ACBD3 is a Golgi resident protein involved in the maintenance of the Golgi structure and regulation of intracellular trafficking between the endoplasmic reticulum and the Golgi. However, in enterovirus-infected cells, the ACBD3 GOLD domain interacts preferentially with viral non-structural 3A proteins, which causes re-localization of ACBD3 to the sites of virus replication. In this study, we present a structural, biochemical, and biological characterization of the complexes composed of human ACBD3 and the 3A proteins of four representative enteroviruses. The crystal structures revealed the details of the ACBD3-3A interaction, the 3A-3A interaction causing the assembly of the ACBD3-3A heterotetramers, the interaction between the ACBD3-3A complex and the lipid bilayer, and the roles of these interactions in facilitation of enterovirus replication.

To ensure that the 3A protein is fully complexed with the ACBD3 GOLD domain and to avoid the formation of partial complexes with 1:2 stoichiometry, we designed a GOLD-EVD68 3A fusion protein using a similar approach as for the GOLD-EVA71 3A fusion protein used for the crystallographic analysis. Taking advantage of the vicinity of the C terminus of the ACBD3 GOLD domain and the N terminus of the ordered part of the EVD68 3A protein, we connected the last residue of ACBD3 (R528ACBD3) through a short peptide linker (GSGSG) to the first ordered residue of the EVD68 3A protein (T163A/EVD68). Both GOLD-3A wild-type and LVVY mutant fusion proteins formed crystals, which diffracted to a resolution suitable for further structure determination. The crystal structures of the GOLD: 3A complex consisting of two individual proteins, the GOLD-3A fusion protein, and its LVVY mutant were almost identical with low root-median-square deviations, confirming that neither the fusion-protein approach nor the LVVY mutation affected the correct folding of these proteins. Three lines of evidence document the dimeric state of the wild-type GOLD-3A fusion protein and the monomeric state of its LVVY mutant in vitro. First, the retention volumes of these proteins in size exclusion chromatography are significantly shifted. Secondly, the small-angle X-ray scattering (SAXS) profiles of these proteins correspond to the calculated scattering curves of a dimer of the wild-type GOLD-3A fusion protein and of a monomer of its LVVY mutant. Nevertheless, we observed a significant difference in FRET efficiency between the wild-type GOLD-3A fusion protein and its LVVY mutant. These results confirm that the GOLD: 3A complexes are flexible enough to allow the formation of the heterotetramers consisting of two molecules of the viral 3A protein and two molecules of host ACBD3 even in cells at the respective intracellular membranes.

> GAMESLPVIAAPSMWTRPQIKDFKEKIQQDADSVITVGRGEVVTVRVPTHEEGSYLFWEFATDNYDIGFGVYFEWTDSPNTAVSVHVSESSDDDEEEEENIGCEEKAKKNANKPLLDEIVPVYRRDCHEEVYAGSHQYPGRGVYLLKFDNSYSLWRSKSVYYRVYYTR;> GSGSGTPAPDAINDLLRSVDSQEVRDYCQKKGWIVIHPSNELVVEKHISR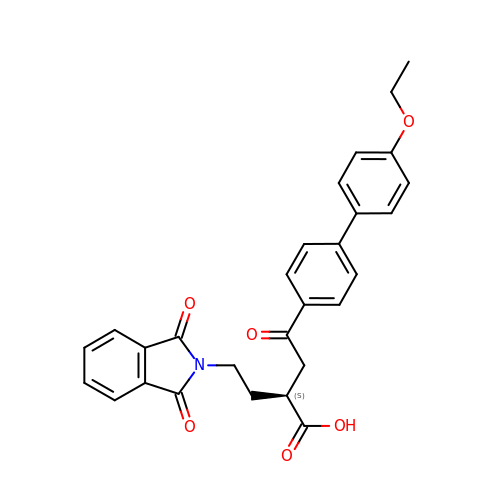2-[2-(1,3-DIOXO-1,3-DIHYDRO-2H-ISOINDOL-2-YL)ETHYL]-4-(4'-ETHOXY-1,1'-BIPHENYL-4-YL)-4-OXOBUTANOIC ACID | C28 H25 N O6 | AQYSXARQCHHHLK-NRFANRHFSA-N> MTTHIFHADDLLQALQQAKAEKNFSSVFSLDWDKLRTAKRNTTVKYVTVNVIVKGKKAPLMFNFQNEKHVGTIPPSTDEEVI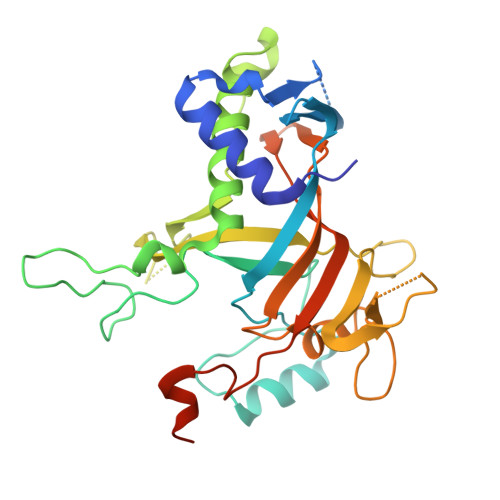RMNAENPKFLVKKRDRDPCLQFNKYKISPPLEDDGLTVKKNEQGEEIYPGDEEKSKLFQIIELLEEAFEDAVQKGPEAMKTKHVIKLIQRKISNSAVKNADKPLPNPIARIRIKINPATSILTPILLDKNKPITLQNGKTSFEELKDEDGVKANPDNIHKLIESHSIHDGIINARSICISNMGISFPLCLEMGVVKVFEKNNGIDVNSIYGSDDISTLVNQIAIA N-ETHYLHYDROXY-DOXORUBICIN 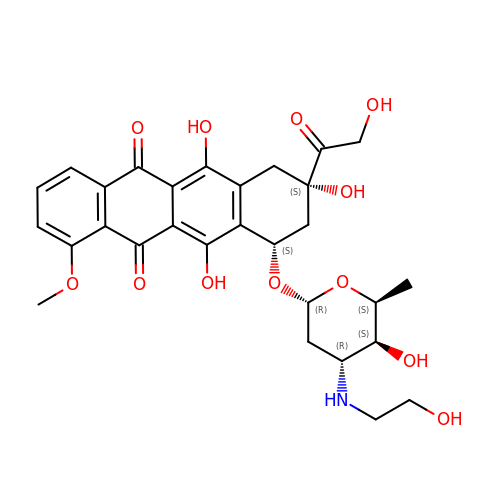| C29 H33 N O12 | XZJOMGCCXRRFJX-MIDWVNFUSA-N>[2x]SNVPHKSSLPEGIRPGTVLRIAGLVPPNASRFHVNLLCGEEQGSDAALHFNPRLDTSEVVFNSKEQGSWGREERGPGVPFQR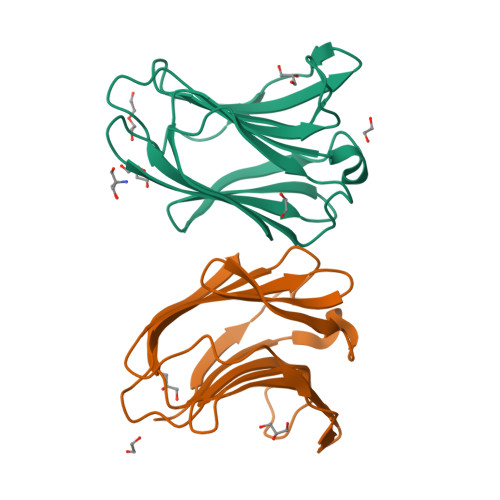GQPFEVLIIASDDGFKAVVGDAQYHHFRHRLPLARVRLVEVGGDVQLDSVRIF2-[[2-methoxy-4-(2-oxidanylidenepyrrolidin-1-yl)phenyl]amino]-4-(methylamino)-7H-pyrrolo[2,3-d]pyrimidine-5-carbonitrile | C19 H19 N7 O2 | 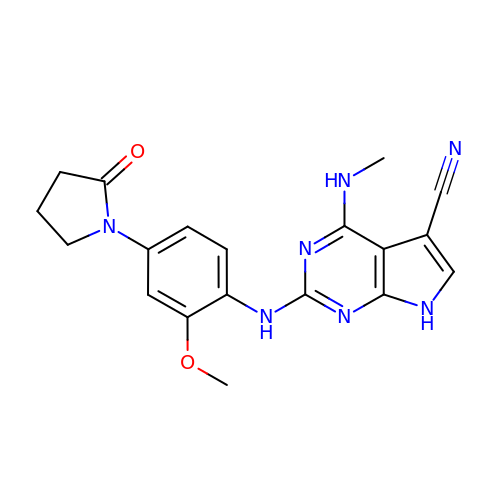MOBTUTZGYGGLCO-UHFFFAOYSA-N> MSSVNFDISMANFAMELYRQSFSNQS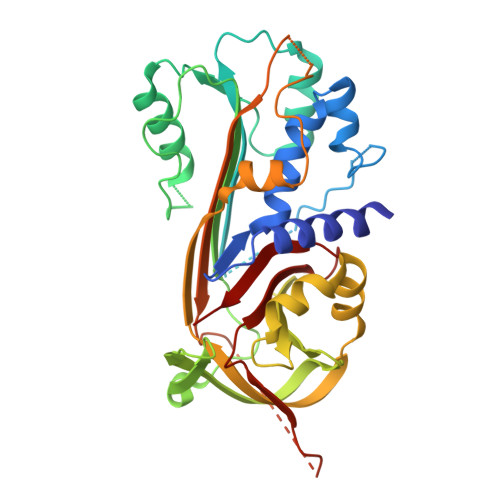NSFFSPYSIVLTLAMTYFGSSGRTKQQLKDRLFSVSDDQLQASLDGIFQSLQGDQHQQEQLTMQLHLANRLFARNNLKLLPAYLTRIQKTFKADVDLVDFSNGAAAAEKINRWVANETKDRIKNLIPPDVLDEMTCLVLVNAIYFKGNWQTRFAPESTSKQYFSVDQNTNKLVDMMHVNDTFRHAEHEQFQILQLPYESSKLAMYVLLPKEKFGLEKLVNQLSGEQLLDSMEAVTSKKVSITFPKFKLEETLPLKKILLQLGLTSMFDHSMADFSMMTGDRSVIVSDAFHKAFIEVNEEGSEASAATAVVAMLRSAQHVAPPAVFIADHPFMFLIADMQTQTILFMGSYRG>[4x]MVLMIVSGRSGSGKSVALRALEDMGFYCVDNLPVVLLPDLARTLADREISAAVSIDVRNMPESPEIFEQAMSNLPDAFSPQLLFLDADRNTLIRRYSDTRRLHPLSSKNLSLESAIDKESDLLEPLRSRADLIVDTSEMSVHELAEMLRTRLLGKRERELTMVFESFGFKHGIPIDADYVFDVRFLPNPHWDPKLRPMTGLDKPVAAFLDRHTEVHNFIYQTRSYLELWLPM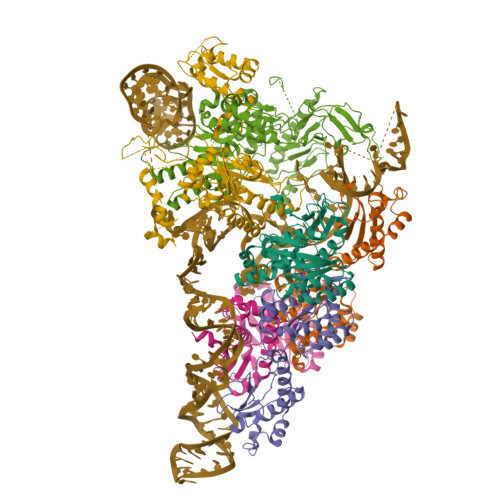LETNNRSYLTVAIGCTGGKHRSVYIAEQLADYFRSRGKNVQSRHRTLEKRKP;>[2x]MKRMLINATQQEELRVALVDGQRLYDLDIESPGHEQKKANIYKGKITRIEPSLEAAFVDYGAERHGFLPLKEIAREYFPANYSAHGRPNIKDVLREGQEVIVQIDKEERGNKGAALTTFISLAGSYLVLMPNNPRAGGISRRIEGDDRTELKEALASLELPEGMGLIVRTAGVGKSAEALQWDLSFRLKHWEAIKKAAESRPAPFLIHQESNVIVRAFRDYLRQDIGEILIDNPKVLELARQHIAALGRPDFSSKIKLYTGEIPLFSHYQIESQIESAFQREVRLPSGGSIVIDSTEALTAIDINSARATRGGDIEETAFNTNLEAADEIARQLRLRDLGGLIVICFIDMTPVRHQRAVENRLREAVRQDRARIQISHISRFGLLEMSRQRLSPSLGESSHHVCPRCSGTGTVRDNESLSLSILRLIEEEALKENTQEVHAIVPVPIASYLLNEKRSAVNAIETRQDGVRCVIVPNDQMETPHYHVLRVRKGEETPTLSYMLPKLHEEAMALPSEEEFAERKRPEQPALATFAMPDVPPAPTPAEPAAPVVAPAPKAAPATPAAPAGGEETKPTEQPAPKA> MFGIGTKDLGIDLGTANTLVYVKGKGIVLREPSVVAIQRDTKQIVAVGNEAKNMIGRTPGNIVALRPMKDGVIADYETTATMMKYYIRKAIKTKGLFAGKPYVMVCVPYGITAVEERAVIDATRQAGARDAYTIEEPFAAAIGANLPVWEPTGSMVVDIGGGTTEVAVISLGGIVTSQSIRIAGDEMDEAIIQYIRKSYNLMIGERTAEAIKMEIGSAGNPEGIGNMEIRGRDLLTGLPKTIEISAEEVAEALRDTVYAIVESVKNTLEKTPPELAADIMDRGIVLTGGGALLRNLDKVISQETDMPVIVAENPLDCVAIGTGKALDHIDLFKNKARDHR

In vivo, MreB proteins form discrete, nanometer-long, membrane-associated polymeric assemblies along the cell cylinder that move processively around the rod circumference together with proteins of the cell wall (CW) elongation machinery, forming the so-called Rod complex. The current model is that self-aligned MreB filaments restrict the diffusion of CW biosynthetic proteins in the membrane and orient their motion to insert new peptidoglycan strands in radial hoops perpendicular to the long axis of the cell, promoting the cylindrical expansion of rod-shaped cells. We successfully purified a soluble form of MreB from the Gram-positive thermophilic Geobacillus stearothermophilus (MreBGs) and elucidated its crystal structure, confirming the classical actin/MreB fold and the presence of the small hydrophobic loop shown to mediate membrane binding in MreBTm and MreB5Sc. We also show that the interaction with lipids is mediated by electrostatic interactions and by two spatially close hydrophobic motifs in the MreBGs monomers that comprise the small hydrophobic loop and the N-terminal end.

The crystals belong to the monoclinic P21 space group and contain one molecule of MreBGs per asymmetric unit. Monomers of apo MreBGs display the canonical fold of actin-like proteins, characterized by four subdomains IA, IIA, IB and IIB. Subdomain IA (blue) of MreBGs is formed by residues 1–32, 66–145 and 315–347; subdomain IB (yellow) by residues 33–65; IIA (red) by residues 146–181 and 246–314 and IIB (green) by residues 182–245. Loop β6-α2, which connects subdomains IA and IB and closes the nucleotide-binding pocket, is partially disordered in apo MreBGs. In domain IA, the hydrophobic loop α2-β7, which has been shown to be involved in MreBTm membrane binding and is 2 residues longer in MreBGs, displays a distinct conformation, packed on the N-terminal extremity of the polypeptide chain. Crystal packing analysis revealed straight protofilaments characterized by a subunit repeat distance of 51 Å, similar to that observed in crystal structures of other actin homologs. However, because of the open conformation of MreBGs, domain IB interacts with domain IA and not with domain IIA as observed for example for MreBTm (van den Ent et al., 2001). We noticed that in the crystal structure of the apo form of MreBGs this short hydrophobic N-terminal sequence is in close proximity to loop α2-β7, which in MreBTm carries the hydrophobic residues L93 and F94 involved in membrane binding. Interestingly, analysis of the crystal structure of MreBGs also showed that a cluster of positively charged residues surrounds the protruding hydrophobic subdomain formed by the α2-β7 loop and the N-terminal sequence.>MTSASSPPAFRLETSDGDEEGNAEVNKGKQEPPPMESPFQREDRNSSPQIKVNLNFIKRPPKNTSAPSQQEPDRFDRDRLFSVVSRGVPEELTGLLEYLRWNSKYLTDSAYTEGSTGKTCLMKAVLNLQDGVNACIMPLLQIDKDSGNPKLLVNAQCTDEFYQGHSALHIAIEKRSLQCVKLLVENGADVHLRACGRFFQKHQGTCFYFGELPLSLAACTKQWDVVTYLLENPHQPASLEATDSLGNTVLHALVMIADNSPENSALVIHMYDGLLQMGARLCPTVQLEEISNHQGLTPLKLAAKEGKIEIFRHILQREFSGPYQPLSRKFTEWCYGPVRVSLYDLSSVDSWEKNSVLEIIAFHCKSPNRHRMVVLEPLNKLLQEKWDRLVSRFFFNFACYLVYMFIFTVVAYHQPSLDQPAIPSSKATFGESMLLLGHILILLGGIYLLLGQLWYFWRRRLFIWISFMDSYFEILFLLQALLTVLSQVLRFMETEWYLPLLVLSLVLG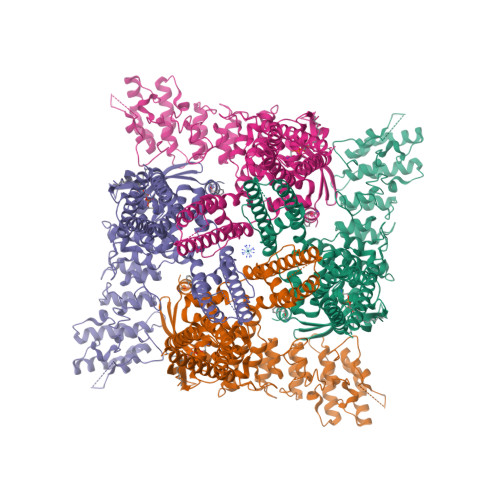WLNLLYYTRGFQHTGIYSVMIQKVILRDLLRFLLVYLVFLFGFAVALVSLSREARSPKAPEDNNSTVTEQPTVGQEEEPAPYRSILDASLELFKFTIGMGELAFQEQLRFRGVVLLLLLAYVLLTYVLLLNMLIALMSETVNHVADNSWSIWKLQKAISVLEMENGYWWCRRKKHREGRLLKVGTRGDGTPDERWCFRVEEVNWAAWEKTLPTLSEDPSGPGITGNKKNPTSKPGKNSASEEDHLPLQVLQSP[4x]> GSALSPPRRKAFKKWTPPRSPFNLVQETLFHDPWKLLIATIFLNRTSGKMAIPVLWKFLEKYPSAEVARTADWRDVSELLKPLGLYDLRAKTIVKFSDEYLTKQWKYPIELHGIGKYGNDSYRIFCVNEWKQVHPE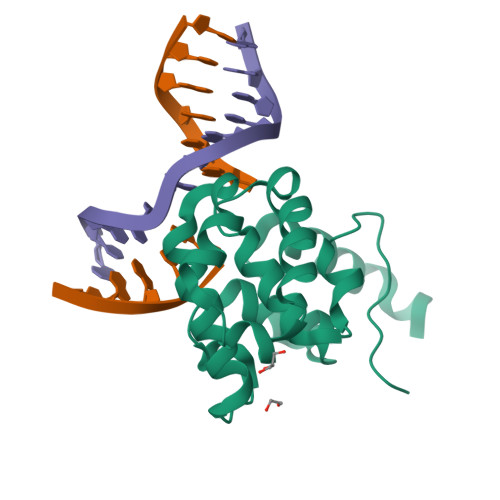DHKLNKYHDWLWENHEKLSLS> APVVNTAYGRVRGVRRELNNEILGPVVQFLGVPYATPPLGARRFQPPEAPASWPGVRNATTLPPACPQNLHGALPAIMLPVWFTDNLEAAATYVQNQSEDCLYLNLYVPTEDGPLTKKRDEATLNPPDTDIRDSGKKPVMLFLHGGSYMEGTGNMFDGSVLAAYGNVIVATLNYRLGVLGFLSTGDQAAKGNYGLLDQIQALRWLSENIAHFGGDPERITIFGSGAGASCVNLLILSHHSEGLFQKAIAQSGTAISSWSVNYQPLKYTRLLAAKVGCDREDSTEAVECLRRKSSRELVDQDVQPARYHIAFGPVVDGDVVPDDPEILMQQGEFLNYDMLIGVNQGE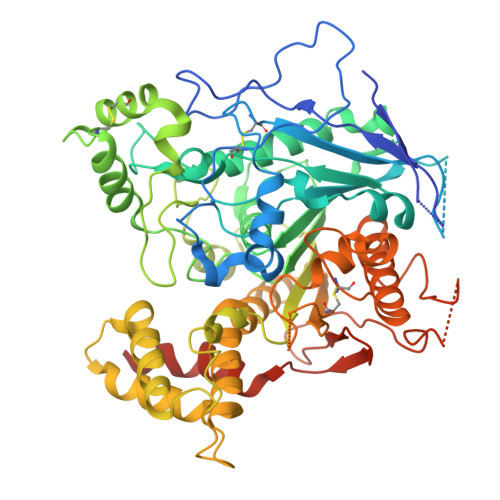GLKFVEDSAESEDGVSASAFDFTVSNFVDNLYGYPEGKDVLRETIKFMYTDWADRDNGEMRRKTLLALFTDHQWVAPAVATAKLHADYQSPVYFYTFYHHCQAEGRPEWADAAHGDELPYVFGVPMVGATDLFPCNFSKNDVMLSAVVMTYWTNFAKTGDPNQPVPQDTKFIHTKPNRFEEVVWSKFNSKEKQYLHIGLKPRVRDNYRANKVAFWLELVPHLHNLHASTSHHHHHH When building atomic models into weak and/or low-resolution density, a common strategy is to restrain their conformation to that of a higher resolution model of the same or similar sequence. When doing so, it is important to avoid over-restraining to the reference model in the face of disagreement with the experimental data. Here, two new such potentials are described: a Cartesian distance restraint derived from a recent generalization of common loss functions and a periodic torsion restraint based on a renormalization of the von Mises distribution. Further, their implementation as user-adjustable/switchable restraints in ISOLDE is described and their use in some real-world examples is demonstrated.

Manual checking and (where necessary) rebuilding of the reference model is often advisable, particularly for older models; in many cases the output from automatic rebuilding and re-refinement by PDB-REDO may be a better starting point than that downloaded directly from the wwPDB.

> MAHHHHHHSSGLEVLFQGPEPKKYAVTDDYQLSKQVLGLGVNGKVLECFHRRTGQKCALKLLYDSPKARQEVDHHWQASGGPHIVCILDVYENMHHGKRCLLIIMECMEGGELFSRIQERGDQAFTEREAAEIMRDIGTAIQFLHSHNIAHRDVKPENLLYTSKEKDAVLKLTDFGFAKETTQNALQTPCYTPYYVAPEVLGPEKYDKSCDMWSLGVIMYILLCGFPPFYSNTGQAISPGMKRRIRLGQYGFPNPEWSEVSEDAKQLIRLLLKTDPTERLTITQFMNHPWINQSMVVPQTPLHTARVLQEDKDHWDEVKEEMTSALATMRVDYDQV>GEWFKHSETGLKGGGPIDDIRKYIARKSAIKIFNQSINYSATKWPPEPIDKNIHMIWIGTKNISEKNIKLSIDTAKKNPDYNTSIIYDSGISGHEGAKKFMLEKFQDSNVNIIDFRKKSYFSQLKQEPSFAYYEQVIAENKYAQASDILRLLVLKYEGGIYKDIDDIQVKGFGSLTFPKGIGVMREYAPEAGKATAFPNTPIAVTKNNPIINKTLDLAVSNYQRGEKNVLKLAGPDVFTQALYQEIPGLDSKVLNAQLY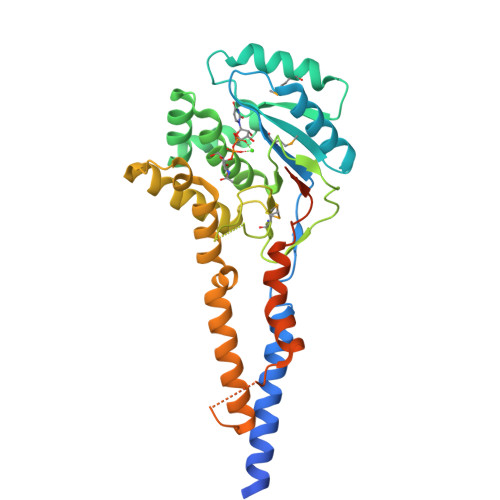QLELAKRQALGVPLEKPKNFADEQLTSAEKEKINRPYQSIRGLSGYVENGADHSWAVDTNIPSTSTQTSTIVTPLAP[2x]> VFHKIRNEDLIFNESLGQGTFTKIFKGVRREVGDYGQLHETEVLLKVLDKAHRNYSESFFEAASMMSKLSHKHLVLNYGVCFCGDENILVQEFVKFGSLDTYLKKNKNCINILWKLEVAKQLAAAMHFLEENTLIHGNVCAKNILLIREEDRKTGNPPFIKLSDPGISITVLPKDILQERIPWVPPECIENPKNLNLATDKWSFGTTLWEICSGGDKPLSALDSQRKLQFY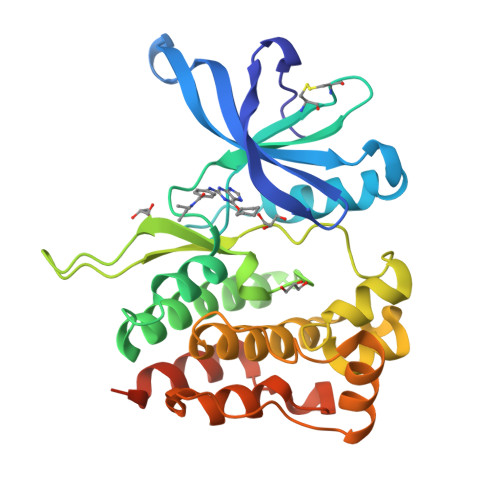EDRHQLPAPKAAELANLINNCMDYEPDHRPSFRAIIRDLNSLFTPDLVPRGSHHHHHH> GAASDEYDYLF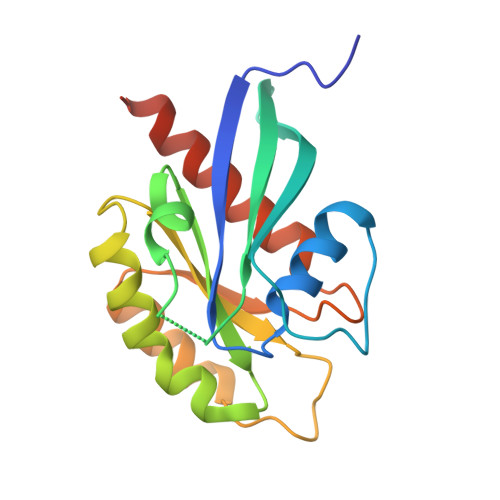KVVLIGDSGVGKSNLLSRFTRNEFNLESKSTIGVEFATRSIQVDGKTIKAQIWDTAGLERYRAITSAYYRGAVGALLVYDIAKHLTYENVERWLKELRDHADSNIVIMLVGNKSDLRHLRAVPTDEARAFAEKNGLSFIETSALDSTNVEAAFQTILTEIYRIVSQKQMSDRRE> MSDQSKPDKAFGEKVRAYLLEHPEVLMEASQKLQEKQAAQQAVSSQKAIGEY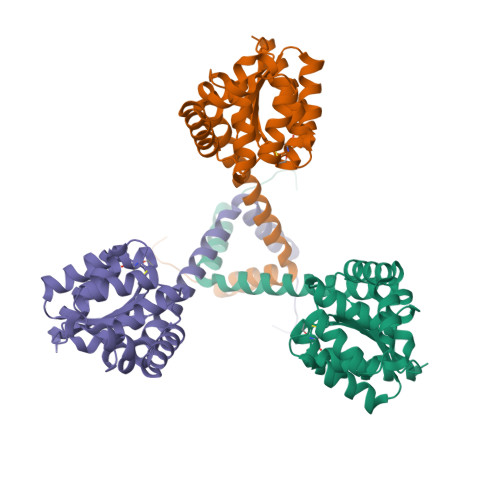RQAIERDPRDIVINPAGTITVTEFFDYRCGYCRQATPAVLELVQKNPDIRLVLKDFVIFGNDSEAAARIALGAKDQGKSLELHKALMAENALDARGALRIAERLGIDMDKAKAVGESQAITQHLADTDALARALNLSGTPAFIVGDTLVPGADIDALKLAIEQTRAARAKAGLEENLYF>GAQDKKKEFKMPTGYAGITHEMSEFYEPVPPVVTPGTDLKGGGFTAPSDAIVLFDGKDLSAWESVKGGAAEWDVHDGVFTVNKKKGDIQTKQKFNDFQMHIEWQVPTNITGESQSRGNSGIFLQGMYEVQVLDCYNNPTYVNGQTGSIYKQSIPLANAMRKPGEWNVYDIIYTAPTFKEDGSYRTHPTVTVIQNGVVLQNHTT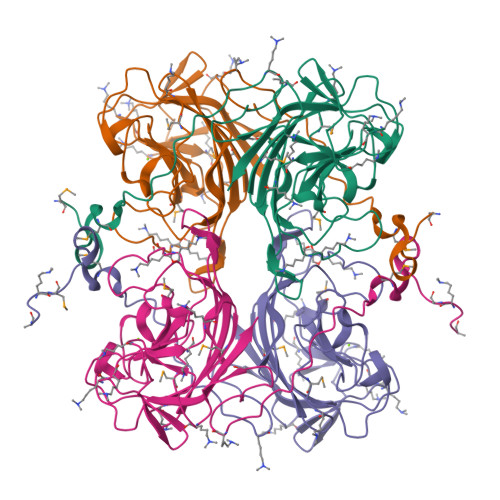ILGTTEWIGFPQVKKHGAGPIILQSHGDPSEPISFRNIWIREL[4x]>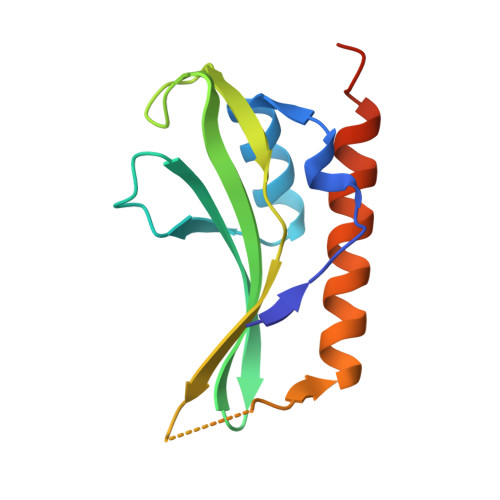[2x]MSLKFENTGLENQTVELSRLDDIMERLGFVRAAQWDYERVTYDRKYVVKEGTYYLRVQGYAIEGNVDSRYALIKLLTPIMGKHYYPHGVEYGDDEHFPSSLVSQCQNVLAQVKSELEKIKEEGHHHHHH((3S,5S)-1,5-dihydroxy-3-methyl-2-oxopyrrolidin-3-yl)phosphonic 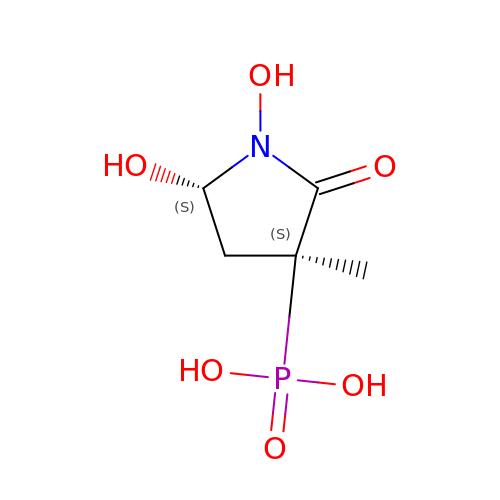acid | C5 H10 N O6 P | VVBLYPMICKYZTP-UCORVYFPSA-N>ADCAKGKIEFSKYNEDNTFTVKVSGREYWTN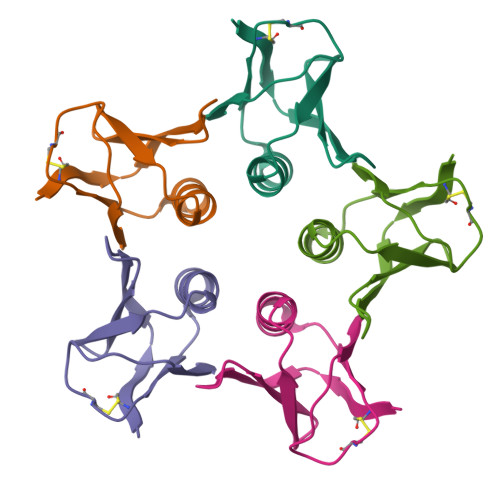RWNLQPLLQSAQLTGMTVTIISNTCSSGSGFAEVQFN[20x]> GDDTQHLTVATLEERPFVIVEPADPISGTCIRDSVPCRSQLNRTHSPPPDAPRPEKRCCKGFCIDILKRLAHTIGFSYD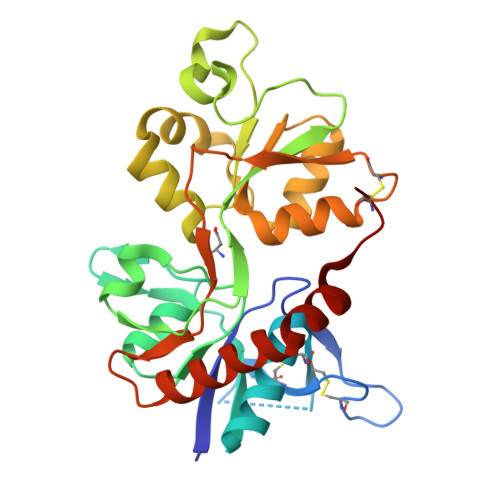LYLVTNGKHGKKIDGVWNGMIGEVFYQRADMAIGSLTINEERSEIVDFSVPFVETGISVMVARGTTVSGLSDRKFQRPQEQYPPLKFGTVPNGSTEKNIRSNYPDMHSYMVRYNQPRVEEALTQLKAGKLDAFIYDAAVLNYMARKDEGCKLVTIGSGKVFATTGYGIALHKGSRWKRPIDLALLQFLGDDEIEMLERLWLSGICHN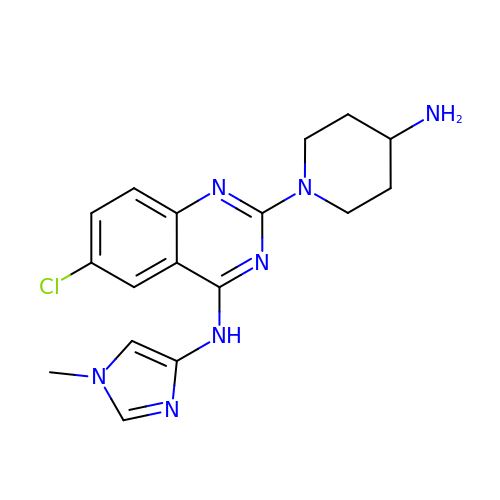2-(4-azanylpiperidin-1-yl)-6-chloranyl-N-(1-methylimidazol-4-yl)quinazolin-4-amine | C17 H20 Cl N7 | FFRWUFYTZPMLTK-UHFFFAOYSA-N~{N}-[(3-chlorophenyl)methyl]-4-ethanoyl-3-ethyl-5-methyl-1~{H}-pyrrole-2-carboxamide | C17 H19 Cl N2 O2 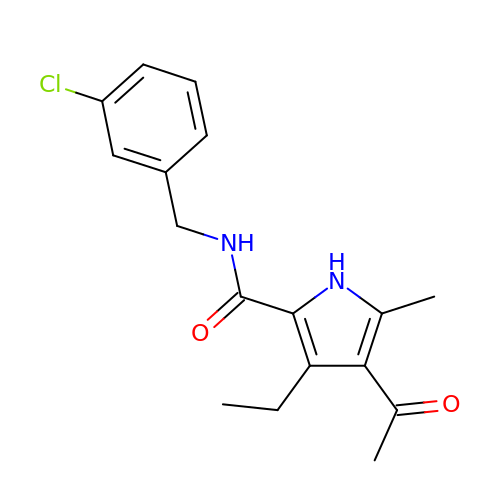| KHTPXNJKROZWBI-UHFFFAOYSA-N> AA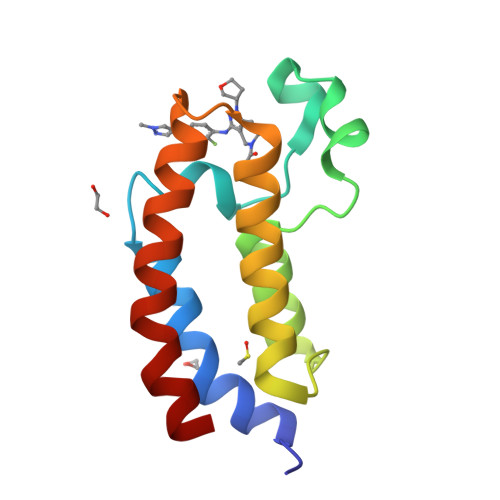FKPEELRQALMPTLEALYRQDPESLPFRQPVDPQLLGIPDYFDIVKNPMDLSTIKRKLDTGQYQEPWQYVDDVWLMFNNAWLYNRKTSRVYKFCSKLAEVFEQEIDPVMQAL>[8x]MADLMMRRGEIWQVDLDPARGSEANNQRPAVVVSNDRANATATRLGRGVITVVPVTSNIAK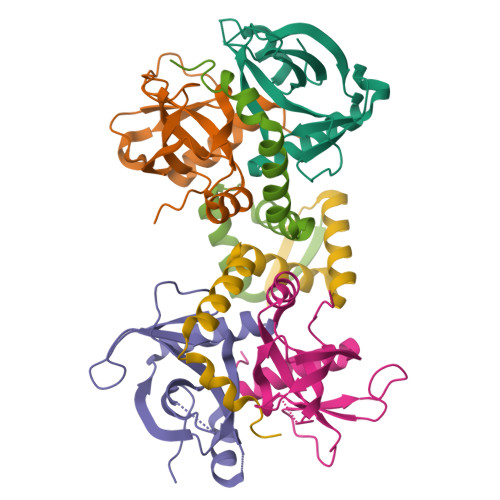VYPFQVLLSATTTGLQVDCKAQAEQIRSIATERLLRPIGRVSAAELAQLDEALKLHLDLWS;>GPSQDPVKLSVSLSDDDVAILDAYVKRAGLPSRSAGLQHAIRVLRYPTLEDDYANAWQEWSAAGDTDAWEQTVGDGVGDAPR[4x]On these grounds, we identified the same enzyme, EUGO from Rhodococcus jostii RHA1, as a promising candidate biocatalyst for the efficient and selective dehydrogenation of dihydrosinapyl alcohol into sinapyl alcohol. This VAO-type enzyme is easy to produce using Escherichia coli, and its crystal structure has been determined. To achieve this, a variant of eugenol oxidase was engineered for the oxidation of dihydrosinapyl alcohol into sinapyl alcohol with good conversion and chemoselectivity. To understand the effects of the introduced mutations in the EUGO8X and EUGO10X, their crystal structures were solved at 2.3 and 1.6 Å resolution, respectively.

The mutations identified from the initial screen, L381Q, S394A, S394V, I427A, and I427V were next individually incorporated into a thermostable variant of EUGO (EUGO S81H A423M H434Y I445D S518P, referred to hereafter as EUGO5X; Tm of 80 °C) that was obtained previously using the FRESCO algorithm. EUGO5X L381Q S394V I427V (“EUGO8X” hereafter) was more selective than EUGO5X L381Q S394V I427A, converting 90% of dihydrosinapyl alcohol with 77% chemoselectivity over 24 h. Despite this, however, the EUGO5X triple mutant was still not a perfect dihydrosinapyl alcohol dehydrogenase. By soaking the crystals with substrate, we obtained the structures in complex with dihydrosinapyl alcohol. Both catalysts contain five stabilizing mutations (S81H, A423M, H434Y, I445D, and S518P), as well as S394V, which have already been discussed in our previous engineering study of EUGO for the dehydrogenation of 4-propylguaiacol. Focusing on the hereby identified activity-improving mutations, the crystal structures show that I427V introduces more space for accommodating the second ortho-methoxy group of dihydrosinapyl alcohol relative to wild-type, explaining the improved conversions allowed by this mutation. L381Q meanwhile forms a new hydrogen bond with the hydroxy group of the substrate side chain, thereby forming a specific substrate–protein interaction. The combined effect of these mutations rationalizes the enhanced activity of the mutant toward dihydrosinapyl alcohol. By superposing the substrate-bound structures of EUGO8X and EUGO10X, a subtle ∼20° rotation of the plane of the aromatic ring and concomitant shift in the position of the propanol side chain of dihydrosinapyl alcohol can be observed.

>[16x]MTRTLPPGVSDERFDAALQRFRDVVGDKWVLSTADELEAFRDPYPVGAAEANLPSAVVSPESTEQVQDIVRIANEYGIPLHPVSTGKNNGYGGAAPRLSGSVIVKTGERMNRILEVNEKYGYALLEPGVTYFDLYEYLQSHDSGLMLDCPDLGWGSVVGNTLDRGVGYTPYGDHFMWQTGLEVVLPQGEVMRTGMGALPGSDAWQLFPYGFGPFPDGMFTQSNLGIVTKMGIALMQRPPASQSFLITFDKEEDLEQIVDIMLPLRINMAPLQNVPVLRNIFMDAAAVSKRTEWFDGDGPMPAEAIERMKKDLDLGFWNFYGTLYGPPPLIEMYYGMIKEAFGKIPGARFFTHEERDDRGGHVLQDRHKINNGIPSLDELQQLDWVPNGGHIGFVPVSAPDGREAMKQFEMVRNRANEYNKDYMAQFVIGLREMYHVCLFIYDTADPEAREEILQMTKVLVREAAEAGYGEYRTHNALMDDVMATFNWGDGALLKFHEKIKDALDPNGIIAPGKSGIWPQRFRGQNL>LDRADILYNIRQTSRPDVIPTQRDRPVAVSVSLKFINILEVNEITNEVDVVFWQQTTWSDRTLAWNSSHSPDQVSVPISSLWVPDLAAYNAISKPEVLTPQLARVVSDGEVLYMPSIRQRFSCDVSGVDTESGATCRIKIGSWTHHSREISVDPTTENSDDSEYFSQYSRFEILDVTQKKNSVTYSCCPEA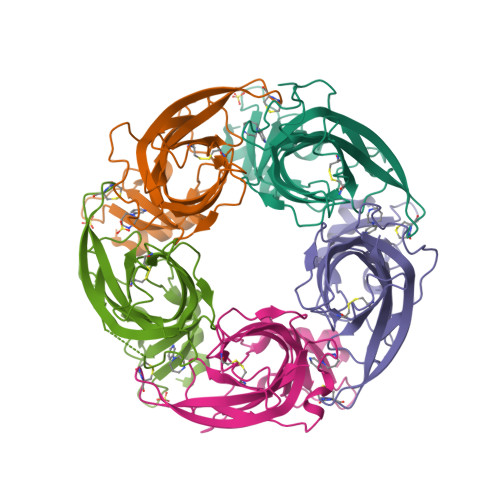YEDVEVSLNFRKKGRSEIL[10x]> GSHMLKDFGKKIKSLRLEKGL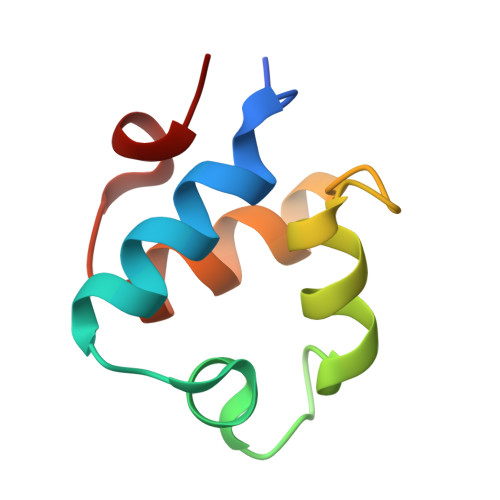TKEAVCLDESQLSTRQLTRIESGQSTPTLNKAVYIAGRLGVTLGYLTD>MSDAVRASDTVFIRETQTPILIERQDNVLFYIRLDAKDSKLLNEVVLDFSKSTPLHDIQSVKLYYGGTEALQHRDKKRMAPVEYISGFHPGTTLSANPSYSVKCAEVVRPSNKVVLKSNYKLFPGVNFFWISLQMKKGTSLYTRINSELCAVKVDGKVLDCKYLSPKNISHRMAIGVRHAGDDGSAAFRIPGLVTTNKGTLLGVYDVRYNSSVDLQEYVDVGLSRSTDGGETWEKMRLPLSFGEYGGLPKAQNGVGDPSILVDTKTNTVWIVAAWTHGMGNQRAWWSSHPGMDMNHTAQLMMVKSTDDGKTWSEPINITEQVKDPSWYFLLQGPGRGITMSDGTLVFPTQFIDSTRIPNAGIMYSKDRGKTWKMHNMARTNTTEAQVVEIEPGVLMLNMRDNRGGSRAVSITKDLGKSWTEHASSRKALNEPVCMASLLNVKAQ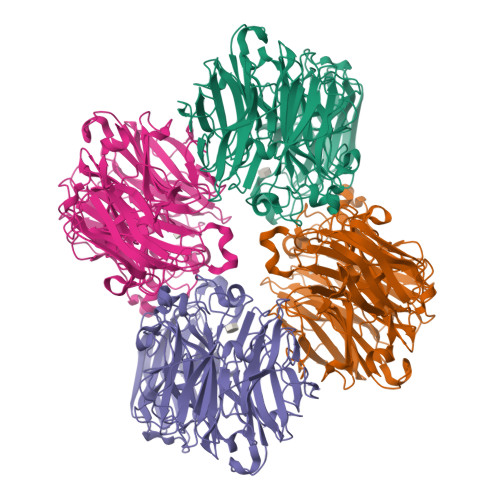DNVLNKDILLFSNPNTVKGRDHITIKASLDKGLTWLPEHQLLLDEDPGWGYSCLTMIDKETIGILYESSVAHMTFQAVKLTDLIKEHHHHHHHHHH[4x]octyl alpha-D-arabinofuranoside | C13 H26 O5 | 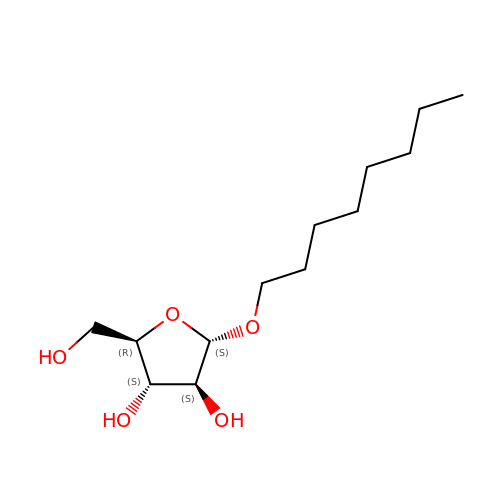DULPXMOVQIYGDB-NDBYEHHHSA-N> SNARDSPYGLSQGITKK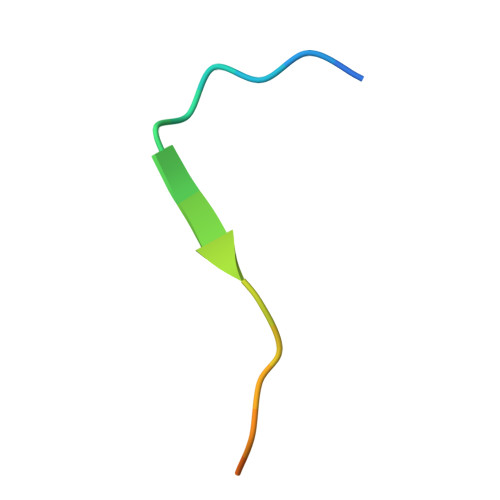NKD> GLEDDLVEVIV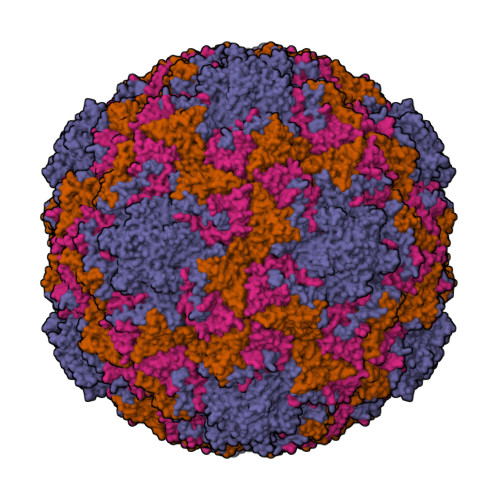DKAQQTLASIKSDSKHTQKVPSLTANETGATLPTTPSDSVETRTTLMHYTGSETTLENFLGRAACVHVVEIVNKRPTDTEEHRMQLLFNNWKINLSSLVQLRRKLEMFTYVRFDSEYTIIATSSQPNEAKFSSNLTIQAMFIPPGAPNPKKWDDYTWQSATNPSVFFNVGKSARFSVPYLGIASAYNCFYDGYSHDNSTTPYGINVLNHMGSMAFRVVNEHDNHTTHVKVRVYHRAKHIRAWVPRAPRALEYLHIGRTNYKQSPQNPIKTRKTISTY;> GYSDRVEQITLGNSTITTQEAANSIVAYGEWPSFLSDVDASDVNKTTKPDTSACRFYTLDSKMWTQGSKGWCWKLPDALKDMGIFGQNMFFHSQGRTGYTIHVQCNATKFHSGCLLVVVIPEHQLASAEGGNVSVLYDKTHPGEKGIDLSEADSTGPMKDPLYMMDGTLIGNSLIFPHQFINLRTNNTATIVVPYINSVPMDSMTRHNNLSLMVIPIVDITATSGTTPSIPVTITIAPMFLELSGIRSKAVI;> GLPTVLTPGSEQFLTTDDRQSPSAMPNYEPTPLIHIPGEVKNLLEIAQVDTLIPLNNTTNTTGLGMYRIPLVQNMQGEQVFGFRLYLGDGVLKTTLLGELCQYFTHWAGSLRLSFMYTGPALSSAKLLIAYTPPGAQGPTKRKEAMLGTHVVWDIGLQSTVVLNIPWTSGVQYRYTDPDTYTSAGFVSCWYQTSLVLPPQTQQTVYMLGFISACPDFKLRLMKDTQSIHQE;> MGAQVSTQKSGSHENQNILTNGSNQTFTVINYYKDAASSSSAGQSFSMDPSKFTEPVKDIMLKGAPALN> GPLGSLCGRVFKVGEPTYSCRDCAVDPTCVLCMECFLGSIHRDHRYRMTTSGGGGFCDCG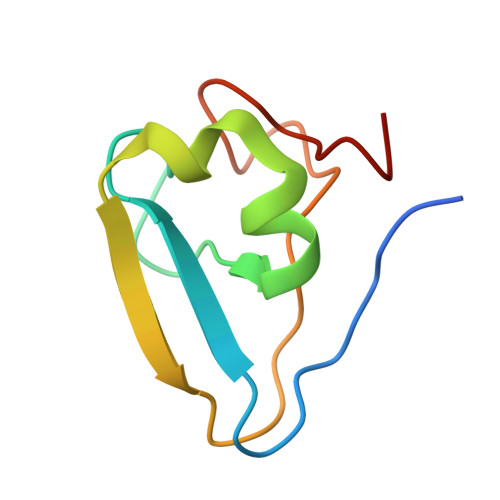DTEAWKEGPYCQKHEL4-[4-(4-aminophenyl)buta-1,3-diyn-1-yl]-N-[(2S,3R)-3-hydroxy-2-methyl-1-nitroso-1-oxobutan-2-yl]benzamide | C22 H19 N3 O4 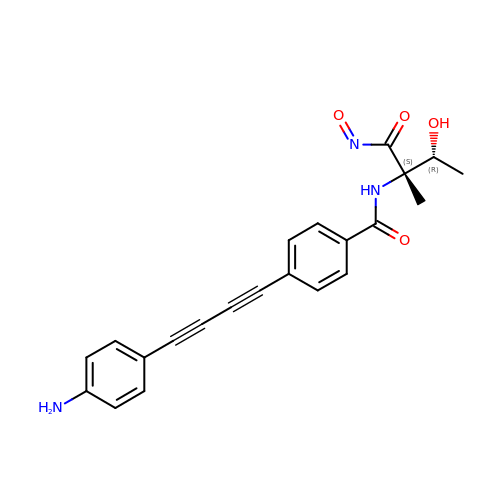| TVYJPPDJMQUKRB-QRQCRPRQSA-N(2R)-3-[2-amino-6-(2-methylphenyl)quinolin-3-yl]-N-[(4R)-2,2-dimethyltetrahydro-2H-pyran-4-yl]-2-methylpropanamide 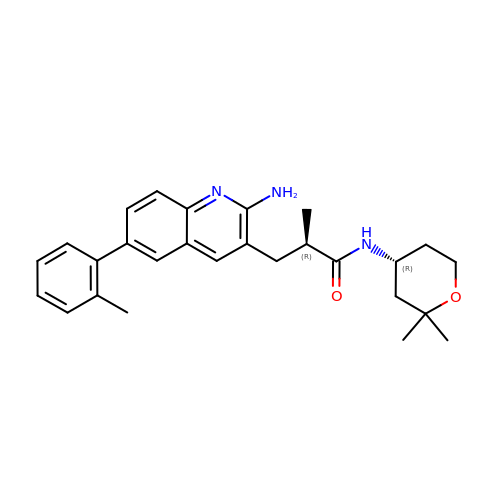| C27 H33 N3 O2 | QMSHBBGXSXAGOO-XMSQKQJNSA-N> MAHHHHHHGHHHQLPTLKVAYIPEHFSTPLFFAQQQGYYKAHDLSIEFVKVPEGSGRLINLLNSNEVDIAIGLTEAFIADIAKGNENIHVLDTYVKSPLLWAVSTGSNRDDVTDAKQLKRIGVSRIGSGSYVMSFVLAHQLGVPSFDQFQVLSNFKNLRDSVNLKDGVEGSDAFMWEYFTSKKYYDNHEIKQ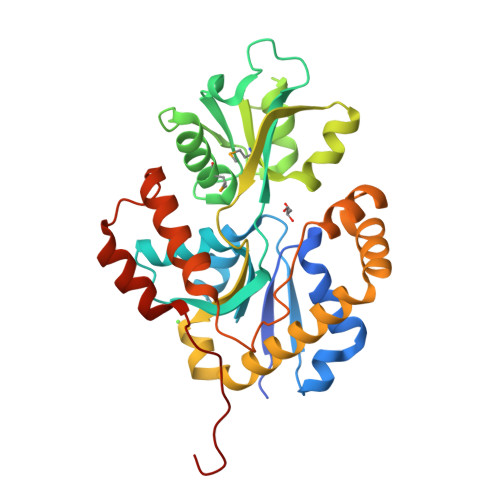IDQIYTPWSSWVVATSSDSLQAKSDVIKNFIDAVNQGIQYYNEHVDEAIEYISSNLDYSAEDAKEWTKTVEFNSRIGKTPLDWDTIVVKTKDTLKLAGVLAESDDVILKRLNSNVKKTNLQLDGDLEAA> MSLGAKPFGEKKFIEIKGRRMAYIDEGTGDPILFQHGNPTSSYLWRNIMPHCAGLGRLIACDLIGMGDSDKLDPSGPERYAYAEHRDYLDALWEALDLGDRVVLVVHDW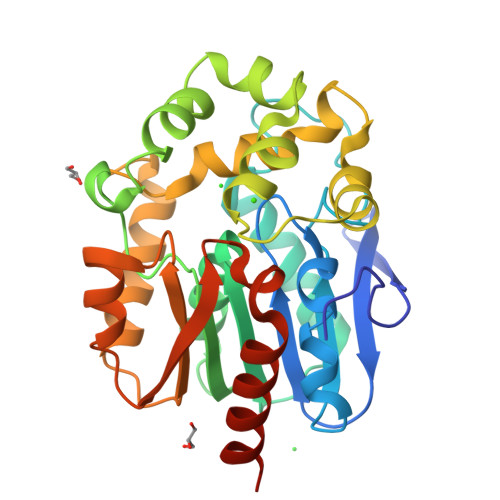GSVLGFDWARRHRERVQGIAYMEAVTMPLEWADFPEQDRDLFQAFRSQAGEELVLQDNVFVEQVLPGLILRPLSEAEMAAYREPFLAAGEARRPTLSWPRQIPIAGTPADVVAIARDYAGWLSESPIPKLFINAEPGHLTTGRIRDFCRTWPNQTEITVAGAHFIQEDSPDEIGAAIAAFVRRLRPAHHHHHH>[3x]MIHLYDAKSFAKLRAAQYAAFHTDAPGSWFDHTSGVLESVEDGTPVLAIGVESGDAIVFDKNAQRIVAYKEKSVKAEDGSVSVVQVENGFMKQGHRGWLVDLTGELVGCSPVVAEFGGHRYASGMVIVTGKGNSGKTPLVHALGEALGGKDKYATVRFGEPLSGYNTDFNVFVDDIARAMLQHRVIVIDSLK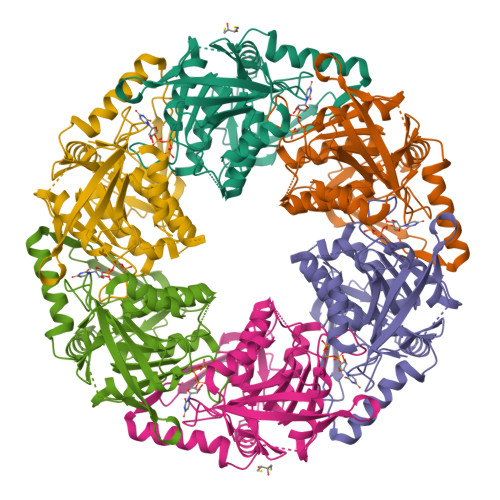NVIGAAGGNTTSGGISRGAFDLLSDIGAMAASRGCVVIASLNPTSNDDKIVELVKEASRSNSTSLVISTDVDGEWQVLTRTGEGLQRLTHTLQTSYGEHSVLTIHTSKQSGGKQASGKAIQTVIKNDELESVLRRLTSN> KLNMLKPDSDLCLKFAMLCTLNDKCDRLRKAYGEACSGPHCQRHVCLRQLLTFFEKAAEPHAQGLLLCPCAPNDRGCGERRRNTIAPNCALPPVAPNCLELRRLCFSDPLCRSRLVDFQTHCHPMDILGTCATEQSRCL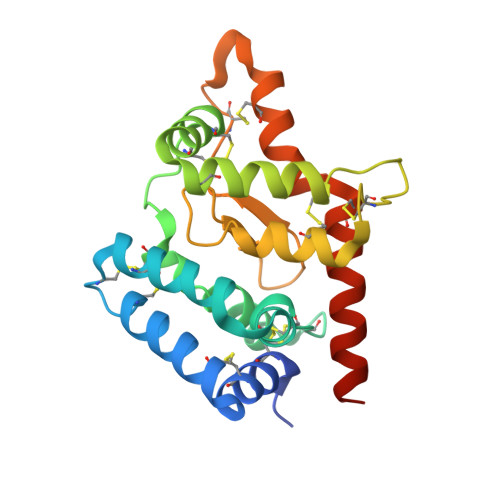RAYLGLIGTAMTPNFVSNVNTSVALSCTCRGSGNLQEECEMLEGFFSHNPCLTEAIAAKMRFHSQLFSQDWPHP>GPLGSQPAERGRNPQVRLLSAEQSMSKVQFRMDNLQFTGVQTSKGVAQVPTFTEGVNISEKGTPILPILSRSLAVSETRAMKVEVVSSKFIEKKDVLIAPSKGVISRAENPDQIPYVYGQSYNEDKFFPGEIATLSDPFILRDVRGQVVNFAPLQYNPVTKTLRIYTEIVVAVSETAEAGQNTISLVKNSTFTGFEDIYKSVFMNYEATR[4x];>[4x]YTPVEEKENGRMIVIVPKKYEEDIEDFVDWKNQRGLRTEVKVAEDIASPVTANAIQQFVKQEYEKEGNDLTYVLLVGDHKDIPAKITPGIKSDQVYGQIVGNDHYNEVFIGRFSCESKEDLKTQIDRTIHYERNITTEDKWLGQALCIASAE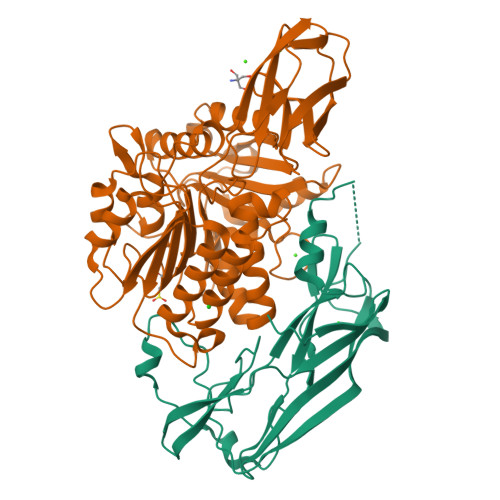GGPSADNGESDIQHENIIANLLTQYGYTKIIKCYDPGVTPKNIIDAFNGGISLANYTGHGSETAWGTSHFGTTHVKQLTNSNQLPFIFDVACVNGDFLYNVPCFAEALMRAQKDGKPTGTVAIIASTINQSWASPMRGQDEMNEILCEKHPNNIKRTFGGVTMNGMFAMVEKYKKDGEKMLDTWTVFGDPSLLVRTLVPTKMQVTAPANISASAQTFEVACDYNGAIATLSDDGDMVGTAIVKDGKAIIKLNESIADETNLTLTVVGYNKVTVIKDVKVEGHHHHHH> GHMSGEAPLTATVDGIIQPMLKAYRIPGMAVAVLKDGKAHYFNYGVANRESGQRVSEQTLFEIGSVSKTLTATLGAYAAVKGGFELDDKVSQHAPWLKGSAFDGVTMAELATYSAGGLPLQFPDEVDSNDKMQTYYRSWSPVYPAGTHRQYSNPSIGLFGHLAANSLGQPFEQLMSQTLLPKLGLHHTYIQVPESAMANYAYGYSKEDKPIRATPGVLAAEAYGIKTGSADLLKFVEANMGYQGDAALKSAIALTHTGFHSVGEMTQGLGWESYDYPVTEQVLLAGNSPAVSFQANPVTRFAVPKAMGEQRLYNKTGSTGGFGAYVAFVPARGIAIVMLANRNYPIEARVKAAHAILSQLAE

Plasmid-based extended-spectrum AmpC enzymes, such as the FOX β-lactamases, are increasingly found in clinical isolates from antibiotic-resistant infections. FOX-4 is of interest because it rapidly hydrolyzes cephamycins. The first generation of BATSIs inactivated serine β-lactamases (Ambler classes A, C, and D) through a dative and reversible covalent bond to the active site serine nucleophile. In this analysis, the structure of FOX-4 in complex with SM23 and LP06, a ceftazidime mimic, is described.

LP06 has the R1 side chain of CAZ and aztreonam. Firstly, LP06 (CAZ analog) solution in DMSO was added to the crystallization drop to bring the inhibitor concentration to 9 mM, and the crystal was frozen after 2 h. The electron density map at a resolution of 1.9 Å shows the LP06 (CAZ analog) molecule covalently attached to S64, but the oxyimino side chain, past the imine nitrogen, is missing. In contrast to the SM23 (CEF analog) complex in which inhibitor binding caused change in the unit cell parameters, the LP06 (CAZ analog) complex has the same unit cell as apo FOX-4. The R1 side chain rings adopt different conformations in FOX-4. In cefoxitin and LP06 (CAZ analog), the ring is perpendicular with Y221 and makes side-to-face π-stacking interactions; in SM23 (CEF analog), it moves out of range. The bulky oxime group, which is missing in the FOX-4 structure, is well resolved in the E. coli AmpC structures with the carboxylate oriented toward its canonical carboxylate binding pocket (N343, R349). The same replacements may account for the disordered oxime side chain of LP06 (CAZ analog), which binds in the same location. It is notable that the cefotaxime-like BATSI shows a slightly lower affinity than LP06 (CAZ analog), suggesting that while the larger oxime side chain of LP06 is disordered, it does contribute somewhat to the overall affinity. LP06 (CAZ analog) mimics the CTX-like BATSI, and binds 2.5-fold more tightly, suggesting that the extended oxime side chain encourages binding.The membrane protein Dispatched (Disp), which belongs to the RND family of small molecule transporters, is essential for Hedgehog (Hh) signaling, by catalyzing the extracellular release of palmitate- and cholesterol-modified Hh ligands from producing cells. Also uniquely among RND proteins, Disp activity requires Furin-mediated cleavage at a conserved site in its first large extracellular domain (ECD1), yielding a mature Disp protein consisting of two non-covalently associated fragments.

Ultimately, a triple-point mutant (hereafter hDisp1NNN) in which three conserved aspartate residues located in transmembrane helices TM4 and TM10 (Asp572, Asp573, and Asp1051) are mutated to asparagine, showed sufficient expression and was well behaved biochemically after purification in detergent; this Disp1 mutant is known to bind Shh stronger than WT Disp1. To this end, we replaced the region in hDisp1 recognized by Furin (residues 263–280) with a cleavage site for the highly specific 3C protease, and we purified to homogeneity the resulting hDisp1NNN-3C protein. Notably, the hDisp1NNN-3C preparation was devoid of the low molecular weight species found in purified hDisp1NNN, indicating that Furin cleavage had been successfully abolished. We solved the structure of uncleaved hDisp1NNN-3C at overall resolution of 3.61 Å, and the structure of hDisp1NNN-3C-cleaved at 3.68 Å. The two ECDs of hDisp1NNN-3C are held together through a helix-swapped configuration, with each ECD accepting secondary structure elements from the other ECD, involving helix α1 of ECD1 and helices α1 and α2 of ECD2. A connecting loop between residues 263–285 in ECD1 (named the C-loop, for protease cleavage) is not well-resolved in our reconstruction, indicating its flexibility; we speculate that this permits its accessibility to Furin or 3C protease cleavage. While the absence of density for the C-loop creates the appearance of a large cavity between the two ECDs, it is important to emphasize that the C-loop, though unstructured, still occupies this space in uncleaved hDisp1NNN-3C (see below). The resolved C-loop is moved away from ECD2 in hDisp1NNN-3C-cleaved, suggesting that the uncleaved C-loop perhaps restricts the motions of the two ECDs, and that proteolytic cleavage allows them to move away from each other. Consistent with this model, extra density was observed at the C-loop position between the two ECDs in the EM map of uncleaved hDisp1NNN-3C at a low contour level, but no extra density was observed at the same position in the map of hDisp1NNN-3C-cleaved at the same or even lower contour level.

> MAMSNGNNDFVVLSNSSIATSAANPSPLTPCDGDHAAQQLTPKEATRTKVSPNGCLQLNGTVKSSFLPLDNQRMPQMLPQCCHPCPYHHPLTSHSSHQECHPEAGPAAPSALASCCMQPHSEYSASLCPNHSPVYQTTCCLQPSPSFCLHHPWPDHFQHQPVQQHIANIRPSRPFKLPKSYAALIADWPVVVLGMCTMFIVVCALVGVLVPELPDFSDPLLGFEPRGTAIGQRLVTWNNMVKNTGYKATLANYPFKYADEQASSLEVLFQGPGSEVDWNFHKDSFFCDVPSDRYSRVVFTSSGGETLWNLPAIKSMCNVDNSRIRSHPQFGDLCQRTTAASCCPSWTLGNYIAILNNRSSCQKIVERDVSHTLKLLRTCAKHYQNGTLGPDCWDMAARRKDQLKCTNVPRKCTKYNAVYQILHYLVDKDFMTPKTADYATPALKYSMLFSPTEKGESMMNIYLDNFENWNSSDGVTTITGIEFGIKHSLFQDYLLMDTVYPAIAIVIVLLVMCVYTKSMFITLMTMFAIISSLIVSYFLYRVVFHFEFFPFMNLTALIILVGIGANNAFVLCDVWNYTKFDKPHAETSETVSITLQHAALSMFVTSFTTAAAFYANYVSNITAIRCFGVYAGTAILVNYVLMVTWLPAVVVLHERYLLNIFTCFKKPQQQIYDNKSCWTVACQKCHKVLFAISEASRIFFEKVLPCIVIKFRYLWLFWFLALTVGGAYIVCINPKMKLPSLELSEFQVFRSSHPFERYDAEYKKLFMFERVHHGEELHMPITVIWGVSPEDNGNPLNPKSKGKLTLDSSFNIASPASQAWILHFCQKLRNQTFFYQTDEQDFTSCFIETFKQWMENQDCDEPALYPCCSHWSFPYKQEIFELCIKRAIMELERSTGYHLDSKTPGPRFDINDTIRAVVLEFQSTYLFTLAYEKMHQFYKEVDSWISSELSSAPEGLSNGWFVSNLEFYDLQDSLSDGTLIAMGLSVAVAFSVMLLTTWNIIISLYAIISIAGTIFVTVGSLVLLGWELNVLESVTISVAVGLSVNFAVHYGVAYRLAPDPDREGKVIFSLSRVGSAMAMAALTTFVAGAMMMPSTVLAYTQLGTFMMLIMCISWAFATFFFQCMCRCLGPQGTCGQIPLPKKLQCSAFSHALSTSPSDKGQSKTHTINAYHLDPRGPKSELEHEFYELEPLASHSCTAPEKTTYEETHICSEFFNSQAKNLGMPVHAAYNSELSKSTESDAGSALLQPPLEQHTVCHFFSLNQRCSCPDAYKHLNYGPHSCQQMGDCLCHQCSPTTSSFVQIQNGVAPLKATHQAVEGFVHPITHIHHCPCLQGRVKPAGMQNSLPRNFFLHPVQHIQAQEKIGKTNVHSLQRSIEEHLPKMAEPSSFVCRSTGSLLKTCCDPENKQRELCKNRDVSNLESSGGTENKAGGKVELSLSQTDASVNSEHFNQNEPKVLFNHLMGEAGCRSCPNNSQSCGRIVRVKCNSVDCQMPNMEANVPAVLTHSELSGESLLIKTL> MARITVEDCLEVVNNRFELVMMASKRARQLANGVQPLIENAAASDKPTVMALREIAAR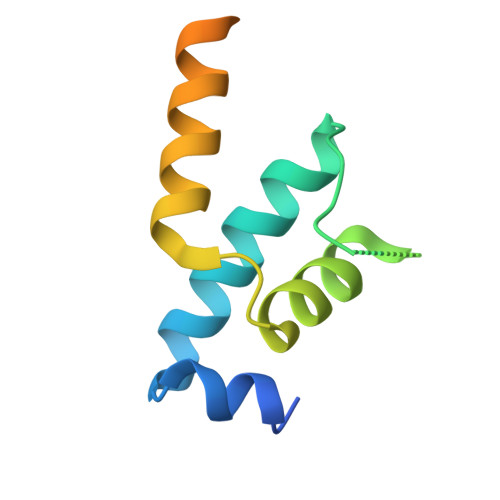RIDNALIDEVEKAERERAEREALEWAAAEVVADEDMSKNDD Expanding this pattern to hpphhph can produce larger α-helical barrels. Here, we show that pentameric to nonameric barrels are accessed by varying the residue at one of the h sites. In peptides with four L/I–K–E–I–A–x–Z repeats, decreasing the size of Z from threonine to serine to alanine to glycine gives progressively larger oligomers. X-ray crystal structures of the resulting α-helical barrels rationalize this: side chains at Z point directly into the helical interfaces, and smaller residues allow closer helix contacts and larger assemblies.

Our hypothesis was that these should direct larger and smaller oligomers, respectively. Encouragingly, the new Thr@g sequences consistently scored best as pentamers: for the a = d = Ile variant the pentameric assembly was favoured outright; while the a = Leu, d = Ile variant scored equally well as pentamer or hexamer. We determined X-ray protein crystal structures for all Gly@g and Thr@g variants. As predicted, the Thr@g peptides formed parallel pentamers (Fig. 3 and Tables S4 and S5†). Significantly, Thr@g with a = d = Ile has a wider channel of ≈9 Å than previous designs (≈7 Å), which increases the scope to functionalize this variant.

>XGEIAQTIKEIAKTIKEIAYTIKEIAQTIKGX[10x]>[6x]SNAMNALAATNRNFKLAARLLGLDSKLEKSLLIPFREIKVECTIPKDDGTLASFVGFRVQHDNARGPMKGGIRYHPEVDPDEVNALAQLMTWKTAVAKIPYGGAKGGIGCDPSKLSISELERLTRVFTQKIHDLIGIHTDVPAPDMGTGPQTMAWILDEYSKFHGYSPAVVTGKPIDLGGSLGRDAATGRGVMFGTEALLNEHGKTISGQRFVIQGFGNVGS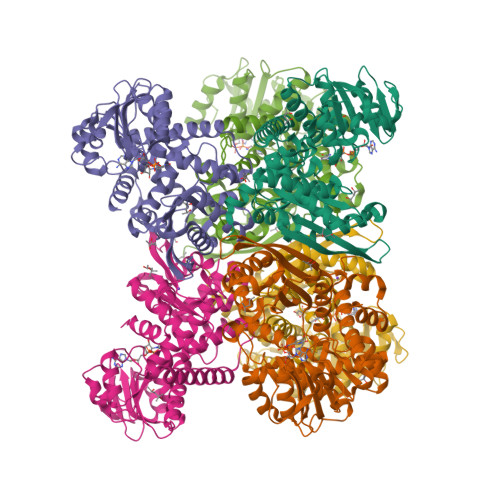WAAKLISEKGGKIVAVSDITGAIKNKDGIDIPALLKHTKEHRGVKGFDGADPIDPNSILVEDCDILVPAALGGVINRENANEIKAKFIIEAANHPTDPDADEILSKKGVVILPDIYANSGGVTVSYFEWVQNIQGFMWEEEKVNDELKTYMTRSFKDLKEMCKTHSCDLRMGAFTLGVNRVAQATILRGWGA>[3x]GPLGSKGVLLKSSISFQNIIEGTRNFHKDFLIGEGEIFEVYRVE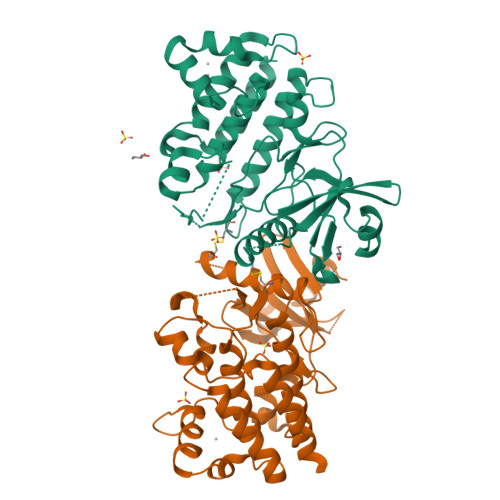IQNLTYAVKLFKQEKKMQCKKHWKRFLSELEVLLLFHHPNILELAAYFTETEKFCLIYPYMRNGTLFDRLQCVGDTAPLPWHIRIGILIGISKAIHYLHNVQPCSVICGSISSANILLDDQFQPKLTDFAMAHFRSHLEHQSCTINMTSSSSKHLWYMPEEYIRQGKLSIKTDVYSFGIVIMEVLTGCRVVLDDPKHIQLRDLLRELMEKRGLDSCLSFLDKKVPPCPRNFSAKLFCLAGRCAATRAKLRPSMDEVLNTLESTQASLYFAE> MKKRKTVKKRYVIALVIVIAGLITLWRILNAPVPTYQTLIVRPGDLQQSVLATGKLDALRKVDVGAQVSGQLKTLSVAIGDKVKKDQLLGVIDPEQAENQIKEVEATLMELRAQRQQAEAELKLARVTYSRQQRLAQTQAVSQQDL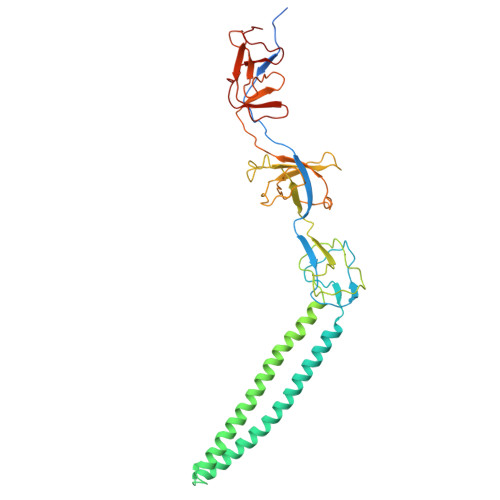DNAATEMAVKQAQIGTIDAQIKRNQASLDTAKTNLDYTRIVAPMAGEVTQITTLQGQTVIAAQQAPNILTLADMSAMLVKAQVSEADVIHLKPGQKAWFTVLGDQLTRYEGQIKDVLPTPEKVNDAIFYYARFEVPNPNGLLRLDMTAQVHIQLTDVKNVLTIPLSALGDPVGDNRYKVKLLRNGETREREVTIGARNDTDVEIVKGLEAGDEVVIGEAKPGAAQ As reported in a companion study, we isolated a cytochrome P450-reductase gene pair, gcoAB, from Amycolatopsis sp. ATCC 39116 (encoding proteins with accession numbers WP_020419855.1 and WP_020419854.1). Unlike other known tetrahydrofolate- or non-heme iron-dependent demethylases, which are fairly substrate specific, the P450-reductase pair characterized here (GcoAB) demethylates diverse aromatic substrates, potentially providing an important advantage in both natural and biotechnological contexts. GcoA and GcoB operate as a multi-domain complex; guaiacol is processed exclusively in GcoA, with electrons supplied by the GcoB redox machinery. While the organization of P450 systems is diverse, the architecture of this 2-protein system, combining a catalytic P450 with a 2Fe-2S ferredoxin domain in addition to FAD and NAD binding sites, represents a new class.

The X-ray crystal structures of GcoA (in complex with guaiacol) and GcoB were determined to resolutions of 1.4 Å and 1.7 Å, respectively. The GcoA structure reveals a typical P450 single-domain architecture with a central heme adjacent to a buried active site, captured with the substrate access loop in the closed position. GcoA possesses a broadly hydrophobic pocket with the two oxygen atoms of the substrate coordinated by backbone carbonyl and amide nitrogen groups from residues Val241 and Gly245, respectively. A series of hydrophobic amino acids is responsible for positioning the aromatic ring, including a triad of phenylalanine residues lining the active site cavity. Close examination of the GcoA-guaiacol active site shows that substrate binding involves interactions between the peptide backbone and the substrate hydroxyl (ring C1) and methoxy groups (C2). The ring C3 position has a relatively close (3.8 Å) interaction with the porphyrin-γ-meso carbon that bridges the propionate-substituted pyrrole rings. Demethylation of guaiacol, which binds tightly to GcoA (KD = 6 nM) was then monitored over time via NADH disappearance at 340 nm under steady-state conditions. In contrast, the free energy profile associated with the opening-closing motion of either GcoA:guaiacol or GcoA:catechol exhibits only one minimum, associated with the closed state, suggesting that the enzyme will close when the substrate or product is bound. The same simulations also suggest that the active site constrains the binding mode of guaiacol, so that the methoxy group points toward and the hydroxyl group is oriented away from the heme iron. This may forestall the lower-energy cyclization reaction pathway predicted for guaiacol by DFT calculations.

> GPMTTTERPDLAWLDEVTMTQLERNPYEVYERLRAEAPLAFVPVLGSYVASTAEVCREVATSPDFEAVITPAGGRTFGHPAIIGVNGDIHADLRSMVEPALQPAEVDRWIDDLVRPIARRYLERFENDGHAELVAQYCEPVSVRSLGDLLGLQEVDSDKLREWFAKLNRSFTNAAVDENGEFANPEGFAEGDQAKAEIRAVVDPLIDKWIEHPDDSAISHWLHDGMPPGQTRDREYIYPTIYVYLLGAMQEPGHGMASTLVGLFSRPEQLEEVVDDPTLIPRAIAEGLRWTSPIWSATARISTKPVTIAGVDLPAGTPVMLSYGSANHDTGKYEAPSQYDLHRPPLPHLAFGAGNHACAGIYFANHVMRIALEELFEAIPNLERDTREGVEFWGWGFRGPTSLHVTWEV>QSLLIGVATSSLALHAPSQIVAAIKSRADQLGASVVVSMVERSGVEACKAAVHNLLAQRVSGLIINYPLDDQDAIAVEAACTNVPALFLDVSDQTPINSIIFSHEDGTRLGVEHLVALGHQQIALLAGPLSSVSARLRLAGWHKYLTRNQIQPIAEREGDWSAMSGFQQTMQMLNEGIVPTAMLVANDQMALGAMRAITESGLRVGADISVVGYDDTEDSSCYIPPLTTIKQDFRLLGQTSVDRLLQLSQGQAVKGNQLLPVSLVKRKTTLAPNTQ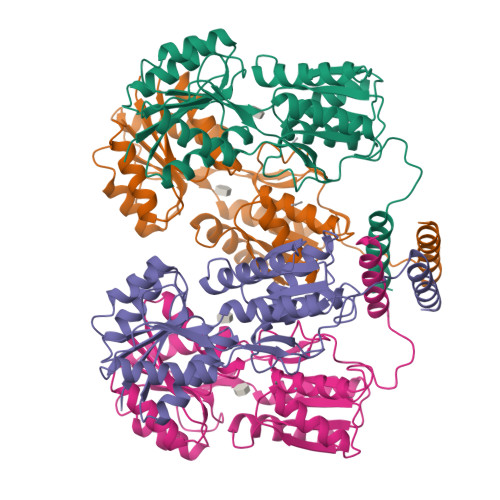TASPRALADSLMQLARQVSRLESGQ[4x]>DNQHKKIKGYRDLSQEEIDMMNRVKELGSQFEKLIQDVSDHLRGQYNASLHNRDEITRIANAEPGRWLAIGKTDIQTGMMAIIRAIAQPDSF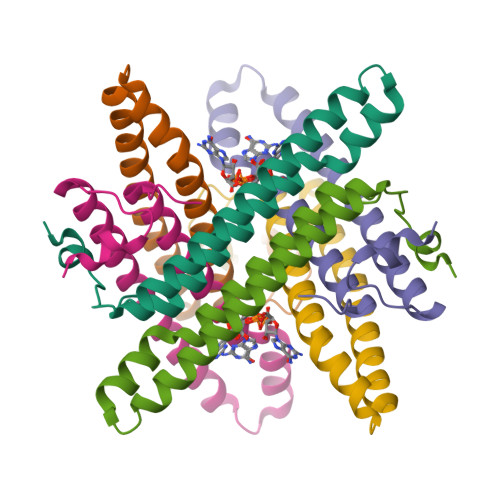[6x]>MSQTLLVHGKDAQGIIKQVLSEVYDAVTSTMGPNGQLVMIKNGVSTKTTKDGVTVARSIRFADEAHELVNRVITEPATKTDEECGDGTTTTIMLTHALYHLFKDFPGFQHHRNIEDLVERVIQRLESMAIRVEVDDPRLYQVALTSSNQDEKLARLVSELYANNKGSYPDIELKEGVNFEDQIEQTTGRTIRMFYANPWFAKGHQGGVTELTGFTAFVIDRRIDKEDTQKLIDGVNHLVKTHKQHLALPILLIARSFEEAANSTLMQLNAAHPTLVEDGRP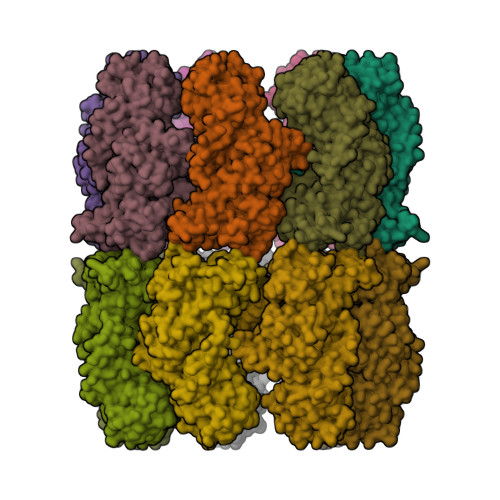WLIPLSTPVGGAIGTSELQDIAVMLNAPMLSDVADLTKLDTHSINGQHGQLELGGNRSILKSTTPKDEDRIEQHARGIEELLEGFSLSDKFSVRARYNERRIRTLRGKLITISVGGETYSEVKERVDRYEDVVKAIRSALENGILPGGGVSLVKAVFGTIKEGLEDKDQSAEFAKRYINSGIANELMRLSTIQHKLLFKDTALYKENGSFHFNDDWLNTPTVMNLATGEIGTPEGLGIYDTAYASITALKGGLQTAKILATTKTLILGEKLSAVKVR[14x]> DSTTEPQTTLHKTITPISGQDDKYELSLDITSKLGTETQTDPLDVVLVADLSGSMQNQDVQSFDGRTISRIDALKNTLRGTNGRKGLIDTILSNSNNRLSMVGFGGKIDNKKVDQYWDGNKWRLFRPYWPYERMTKYYDGVSPWDDANTILGWSNNARAAKTAVYNMSIAGGNSIGTESGIGTGTNIGAGLTLANQLMGSARSNAKKVVILLSDGFANMVYDANGYTIYNYNNEDPNIETAPQWFWDRLNNNLNSLSYSLAPTLDGFYSIKFRYSNNVDSITSLQYYMRQHNASIPNEIFSANDEDQLRDSFKDITDKILPLGIHHVSIKDVLSKYVQLLPNGSSEFRVVKEK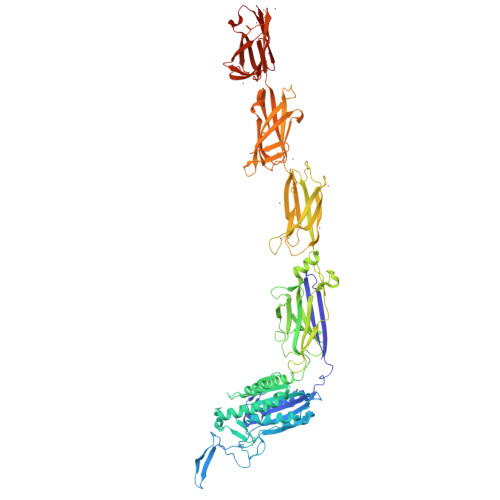DGSSEILTENQVTFDTKTTSEGLVEVTAKFSPNYSLEDGARYVLKFTVTSSQEALDAIAGDKKLEAGDAEGSDVNKLYSNKGASVTYSYGIGNSQTKTKEYSDNPTFKPSDPLTVPVEVEWQGVTGARTVITADQPSNVELKLVQKNKNGGSDNQDYRKTNVNVSKNVSNETRNFEKVAKGYQYDLIAPDVPAFTKEIKNVGTESNPSFKVIYKQLPSLTIKKVLEAENNLNKEFRIKVKLTSPDSKPLNGTFGEITVVNGEAEIRVEKRKRWRGILSYLPRGTHYKVEEEAASTNGYHVTYENQEGDLNKDETSTVTNHKLPSLSVTKKVTGVFANLLKSFKITINIRDAQNSPLNGTYTATVNNKRTPLQFTNGRASIDLNKDQTIKIDGLPLDSHYTVEEETNSSRGYQVSYENQEGKLDGDKSATVTNNKNSVPET>SGFVCNTCPEKWINFQRKCYYFGKGTKQWVHARYACDDMEGQLVSIHSPEEQDFLTKHASHTGSWIGLRNLDLKGEFIWVDGSHVDYSNWAPGEPTSRSQGEDCVMMRGSGRWNDAFCDRKLGAWVCDRL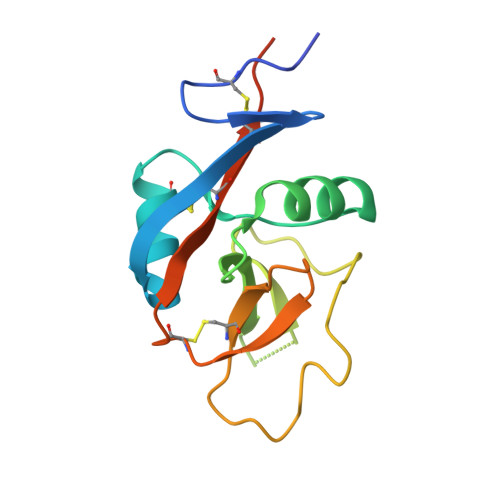ATCTPPASEGSAE[8x]> XPKGRPGPKGFPGYPGPRGRPG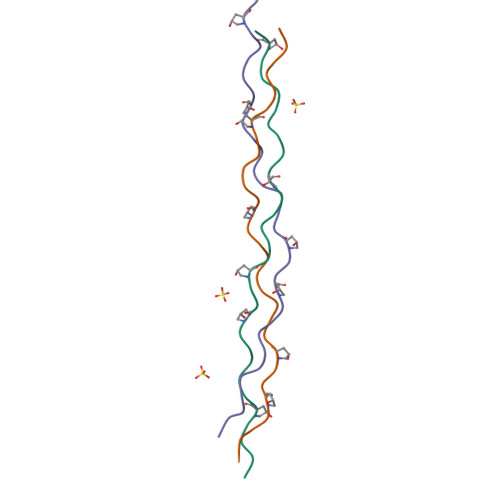KKGPRGPPGX;> XSKGDPGPPGDRGPKGPPGYKGPPGDKGFRGX;> XPDGDRGPRGPPGYPGDDGPEGDPGPPGDPGX>[2x]ATAITYVSKDHYFGRNFDYEISYNEVVTITPRNYKFSFREVGNLDHHFAIIGIAAGIADYPLYYDAINEKGLGMAGLNFSGYADYKKIEEGKENVSPFEFIPWVLGQCSTVDEAKKLLKNLNLVNINFSDELPLSPLHWLLAD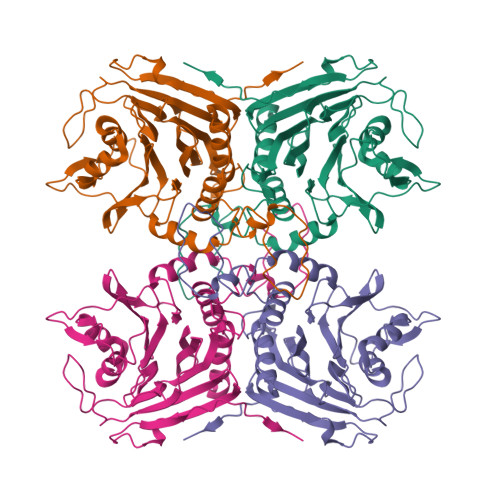KEQSIVVESTKEGLRVFDNPVGVLTNNPTFDYQLFNLNNYRVLSTRTPKNNFSDQIELDIYSRGMGGIGLPGDLSSVSRFVKATFTKLNSVSRSSEYESISQFFHILSSVEQQKGLCDVGDEKYEYTIYSSCCNLEKGIYYYRTYDNSQITAVDMNKENLEKDSLIVYPMVETQQINYAN> GPLGSMATSRYEPVAEIGVGAYGTVYKARDPHSGHFVALKSVRVPNGGGGGGGLPISTVREVALLRRLEAFEHPNVVRLMDVCATSRTDREIKVTLVFEHVDQDLRTYLDKAPPPGLPAETIKDLMRQFLRGLDFLHANCIVHRDLKPENILVTSGGTVKLADFGLARIYSYQMALTPVVVTLWYRAPEVLLQSTYATPVDMWSVGCIFAEMFRRKPLFCGNSEADQLGKIFDLIGLPPEDDWPRDVSL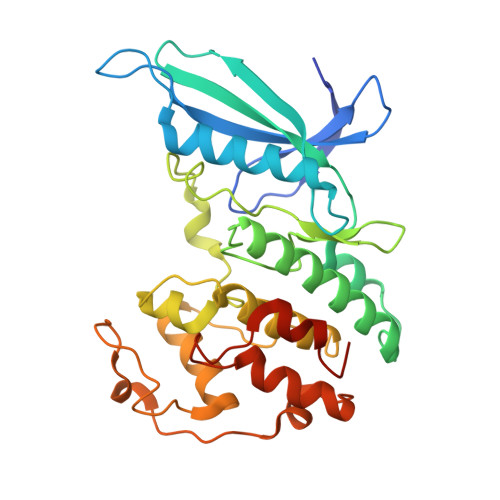PRGAFPPRGPRPVQSVVPEMEESGAQLLLEMLTFNPHKRISAFRALQHSYLHKDEGNPE> MTEIKYKVITKDAFALPYTIIKAKNQPTKGVIVYIHGGGLMFGKANDLSPQYIDILTEHYDLIQLSYRLLPEVSLDCIIEDVYASFDAIQSQYSNCPIFTFGRSSGAYLSLLIARDRDIDGVIDFYGYSRINTEPFKTTNSYYAKIAQSINETMIAQLTSPTPVVQDQIAQRFLIYVYARGTGKWINMINIADYTD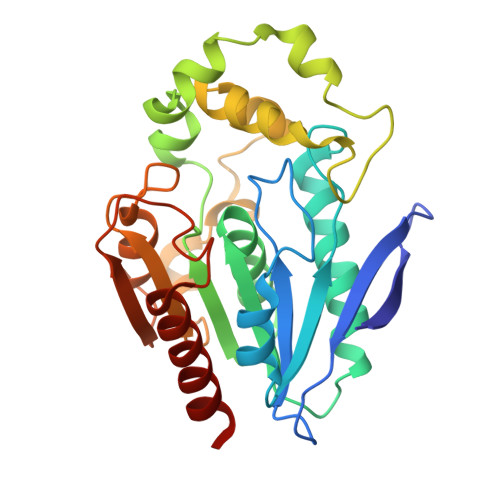SKYNIAPDELKTLPPVFIAHCNGDYDVPVEESEHIMNHVPHSTFERVNKNEHDFDRRPNDEAITIYRKVVDFLNAITMV>ILDGPYQPTTFTPPIDYWILINSNTNGVVYESTNNSDFWTAVVAIEPHVNPVDRQYTVFGENKQFNVRNDSDKWKFLEMFRSSSQNEFYNRRTLTSDTKLVGILKYGGRIWTFHGETPRATTDSSNTANLNDISIIIHSEFYIIP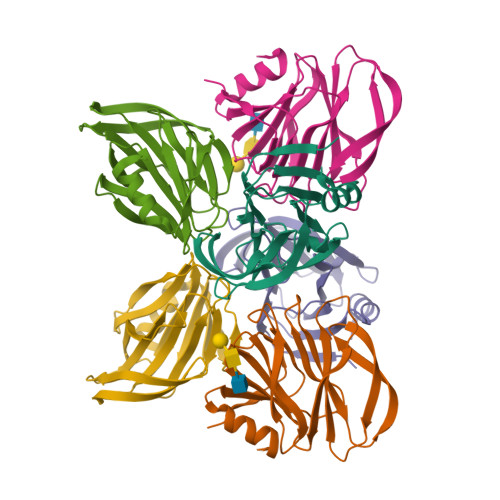RSQESKCNEYINNGL[6x]> GSVGPKTGEENQVLVPNLNPTPENLEVVGDGFKITSSINLVGEEEADENAVNALREFLTANNIEINSENDPNSTTLIIGEVDDDIPELDEALNGTTAENLKEEGYALVSNDGKIAIEGKDGDGTFYGVQTFK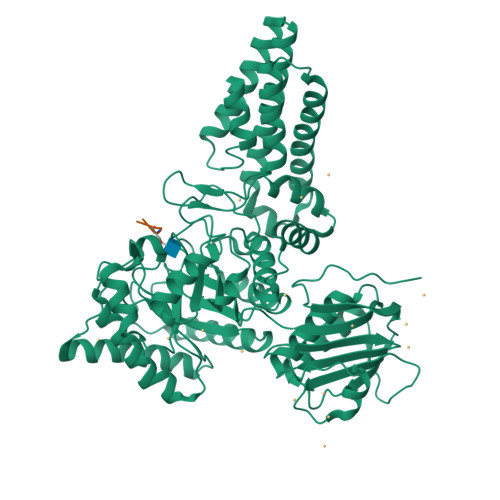QLVKESNIPEVNITDYPTVSARGIVEGFYGTPWTHQDRLDQIKFYGENKLNTYIYAPKDDPYHREKWREPYPESEMQRMQELINASAENKVDFVFGISPGIDIRFDGDAGEEDFNHLITKAESLYDMGVRSFAIYWDNIQDKSAAKHAQVLNRFNEEFVKAKGDVKPLITVPTEYDTGAMVSNGQPRAYTRIFAETVDPSIEVMWTGPGVVTNEIPLSDAQLISGIYDRNMAVWWNYPVTDYFKGKLALGPMHGLDKGLNQYVDFFTVNPMEHAELSKISIHTAADYSWNMDNYDYDKAWNRAIDMLYGDLAEDMKVFANHSTRMDNKTWAKSGREDAPELRAKMDELWNKLSSKEDASALIEELYGEFARMEEACNNLKANLPEVALEECSRQLDELITLAQGDKASLDMIVAQLNEDTEAYESAKEIAQNKLNTALSSFAVISEKVAQSFIQEALS;> VPYSSAQ> MTALDWRSALTADEQRSVRALVTATTAV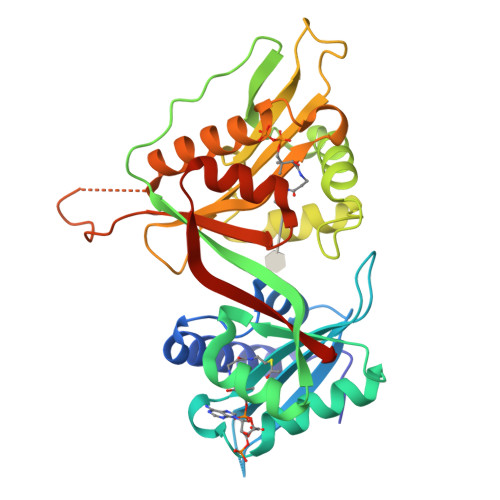DGVAPVGEQVLRELGQQRTEHLLVAGSRPGGPIIGYLNLSPPRGAGGAMAELVVHPQSRRRGIGTAMARAALAKTAGRNQFWAHGTLDPARATASALGLVGVRELIQMRRPLRDIPEPTIPDGVVIRTYAGTSDDAELLRVNNAAFAGHPEQGGWTAVQLAERRGEAWFDPDGLILAFGDSPRERPGRLLGFHWTKVHPDHPGLGEVYVLGVDPAAQRRGLGQMLTSIGIVSLARRLGGRKTLDPAVEPAVLLYVESDNVAAVRTYQSLGFTTYSVDTAYALAGTDN> AAHLSDMLQQLHSVNASKPSERGLVRQEEAEDPACIPIFWVSKWVDYSDKYGLGYQLCDNSVGVLFNDSTRLILYNDGDSLQYIERDGTESYL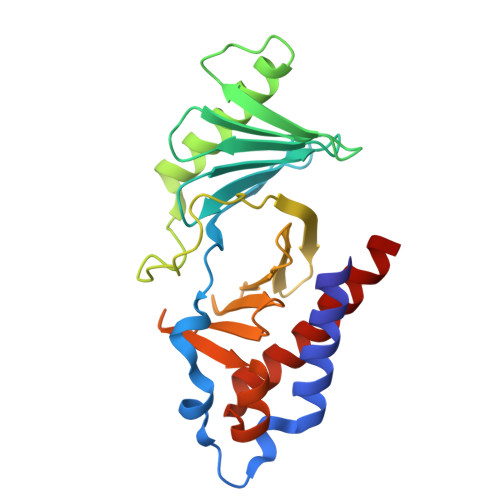TVSSHPNSLMKKITLLKYFRNYMSEHLLKAGANITPREGDELARLPYLRTWFRTRSAIILHLSNGSVQINFFQDHTKLILCPLMAAVTYIDEKRDFRTYRLSLLEEYGCCKELASRLRYARTMVDKLLSSRSA>EELQNKLEDVVIDRNLLILGKILGEGEFGSVMEGNLKQEDGTSLKVAVKTMKLDNSSQREIEEFLSEAACMKDFSHPNVIRLLGVCIEMSSQGIPKPMVILPFMKYGDLHTYLLYSRLETGPKHIPLQTLLKFMVDIALGMEYLSNRNFLHRDLAARNCMLRDDMTVCVADFGLSKKIYSGDYYRQGRIAKM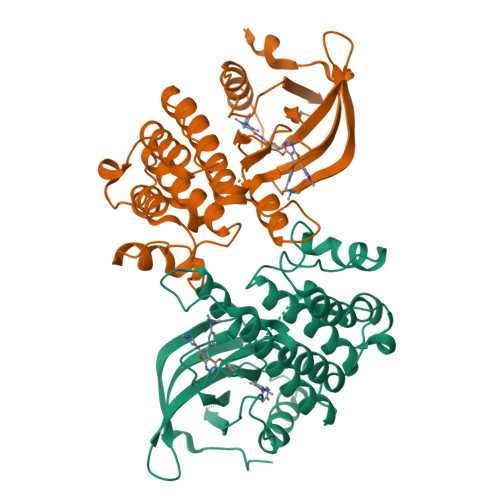PVKWIAIESLADRVYTSKSDVWAFGVTMWEIATRGMTPYPGVQNHEMYDYLLHGHRLKQPEDCLDELYEIMYSCWRTDPLDRPTFSVLRLQLEKLLESLPDV[2x]> TPTLQELKTQLEKGNDETKIETMKRILTIMLNGDPLHGLLMHIIRFVMPSKSKPLKKLLYFYYEICPKLDSQGKLKQEFILVCNGIRNDLQHPNEYIRGNTLRFLCKLREPELLEPLLSSVRACLEHRHAYVRKNAVFAVASIYQHAPSLIPDAADLIATFLEGESDPTC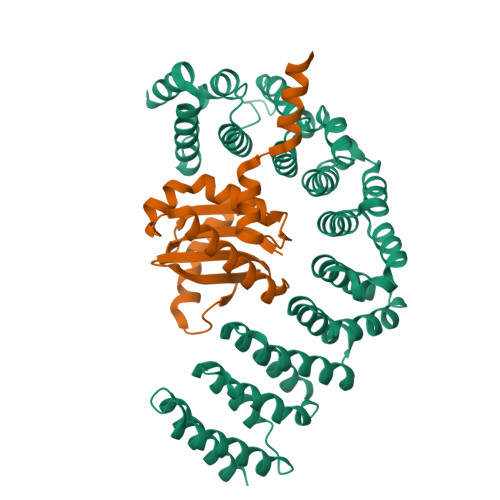KRNGFAALSSISHDKALSYLGTVFEGIPNAEELLQLVEIEFIRKDALHNPQNKPRYLRLIFDLLEANTSTVVYEAASSLTALTNNPVAVKAAAGKFIELAIKEADNNVKLIVLDRVDQLRQKNEGILDDLIMEILRVLSSPDIDVRRKALEIALEMVSSKNVEEVVLLLKKELSKTVEQEYEKNSEYRQLLIHSIHQCAVKFS;> MVVLAASICTRGGKAVLARAFHDIKRSRVEALLASFPKAANSGTQHTTVEQDNVRFVYQPLDELYMVLITNKQSNILQDIDTLHLFAQVVTNTCRTLEEREILRNAYELISAFDEIINLGYRENLTINQIKTFLEMESHEERIQEIIARNKELEATEERKRKAKQLEMQRKEASR>VRIPALERGPGLKDLAIFSRQLATMLGAGLTLLQALAILERQTENRKFREILKQVRTDVEGGMAFSEALS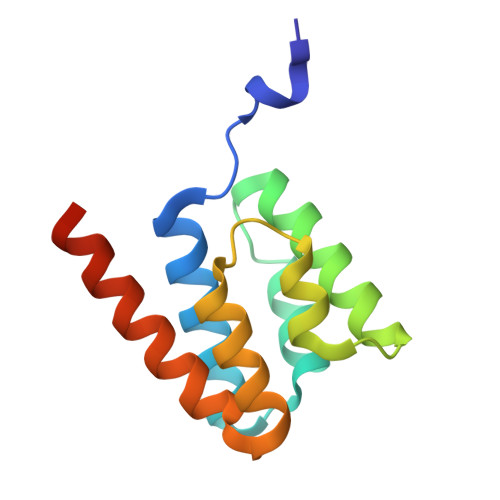KHKIFSRLYVNLVRAGETSGGLDLILDRLASFLEKELELRGKIRSA[2x]> MANNDAVLKRLEQKGAEADQIIEYLKQQVSLLKEKAILQATLREEKKLRVENAKLKKEIEELKQELIQAEIQNGVKQIPFPSGTPLHANSMVSENVIQSTAVTTVSSGTKEQIKGGTGDEKKAKEKIEKKGEKKEKKQQSIAGSADSKPIDVSRLDLRIGCIITARKHPDADSLYVEEVDVGEIAPRTVVSGLVNHVPLEQMQNRMVILLCNLKPAKMRGVLSQAMVMCASSPEKIEILAPPNGSVPGDRITFDAFPGEPDKELNPKKKIWEQIQPDLHTNDECVATYKGVPFEVKGKGVCRAQTMSNSGIK;> MGSSHHHHHHSQDPMMDVLVSECSARLLQQEEEIKSLTAEIDRLKNCGCLGASPNLEQLQEENLKLKYRLNILRKSLQAERNKPTKNMINIISRLQEVFGHAIKAAYPDLENPPLLVTPSQQAKFGDYQCNSAMGISQMLKTKEQKVNPREIAENITKHLPDNECIEKVEIAGPGFINVHLRKDFVSEQLTSLLVNGVQLPALGENKKVIVDFSSPNIAKEMHVGHLRSTIIGESISRLFEFAGYDVLRLNHVGDWGTQFGMLIAHLQDKFPDYLTVSPPIGDLQVFYKESKKRFDTEEEFKKRAYQCVVLLQGKNPDITKAWKLICDVSRQELNKIYDALDVSLIERGESFYQDRMNDIVKEFEDRGFVQVDDGRKI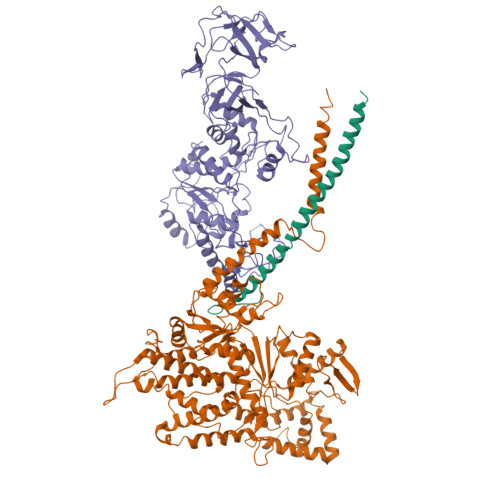VFVPGCSIPLTIVKSDGGYTYDTSDLAAIKQRLFEEKADMIIYVVDNGQSVHFQTIFAAAQMIGWYDPKVTRVFHAGFGVVLGEDKKKFKTRSGETVRLMDLLGEGLKRSMDKLKEKERDKVLTAEELNAAQTSVAYGCIKYADLSHNRLNDYIFSFDKMLDDRGNTAAYLLYAFTRIRSIARLANIDEEMLQKAARETKILLDHEKEWKLGRCILRFPEILQKILDDLFLHTLCDYIYELATAFTEFYDSCYCVEKDRQTGKILKVNMWRMLLCEAVAAVMAKGFDILGIKPVQRM;> HGSSHHHHHHSSGLVPRGSHMASMMAALDSLSLFTSLGLSEQKARETLKNSALSAQLREAATQAQQTLGSTIDKATGILLYGLASRLRDTRRLSFLVSYIASKKIHTEPQLSAALEYVRSHPLDPIDTVDFERECGVGVIVTPEQIEEAVEAAINRHRPQLLVERYHFNMGLLMGEARAVLKWADGKMIKNEVDMQVLHLLGPKLEADLEKKFKVAKARLEETDRRTAKDVVENGETADQTLSLMEQLRGEALKFHKPGENYKTPGYVVTPHTMNLLKQHLEITGGQVRTRFPPEPNGILHIGHAKAINFNFGYAKANNGICFLRFDDTNPEKEEAKFFTAICDMVAWLGYTPYKVTYASDYFDQLYAWAVELIRRGLAYVCHQRGEELKGHNTLPSPWRDRPMEESLLLFEAMRKGKFSEGEATLRMKLVMEDGKMDPVAYRVKYTPHHRTGDKWCIYPTYDYTHCLCDSIEHITHSLCTKEFQARRSSYFWLCNALDVYCPVQWEYGRLNLHYAVVSKRKILQLVATGAVRDWDDPRLFTLTALRRRGFPPEAINNFCARVGVTVAQTTMEPHLLEACVRDVLNDTAPRAMAVLESLRVIITNFPAAKSLDIQVPNFPADETKGFHQVPFAPIVFIERTDFKEEPEPGFKRLAWGQPVGLRHTGYVIELQHVVKGPSGCVESLEVTCRRADAGEKPKAFIHWVSQPLMCEVRLYERLFQHKNPEDPTEVPGGFLSDLNLASLHVVDAALVDCSVALAKPFDKFQFERLGYFSVDPDSHQGKLVFNRTVTLKEDPGKV> SGEKDVVFLIDGSEGVRSGFPLLKDFVQRVVESLDVGPDQVRVALVQYSDRTRPEFYLNSHMDQQGVISAIRRLTLLGGPTPNTGAALEFVLRNILTSSTGSRIAEGVPQLLIVLTAEPSGDDVRGPSVVLKQGGAVPIGIGIGNADISEMQTISFIPDFAVAIPTFRELGTIQQVISERVIQLNREELSSLKPILTPSTGAG

Collagen VI is a ubiquitously expressed extracellular matrix protein that forms a structurally unique network of beaded microfilaments. All collagen VI chains consist of a relatively short triple-helical region as well as of N- and C-terminal globular structures that are largely made up of VWA domains. Von Willebrand factor A (VWA) domains consist of about 200 amino acid residues and act as interaction modules in many intra- and extracellular proteins, e.g., in copines, integrins, von Willebrand factor, complement factors B and C2, matrilins, and collagens. The collagen VI α3N5 domain structure is the first solved structure of a collagen VWA domain and differs from other VWA domains in having an extended C-terminal region comprising residues N1206–G1224.

One of these missense mutations, R1064Q in human (R1064Qh) that is located in the N5 domain, was found in an UCMD patient (Lampe et al., 2005). To gain insight into the UCMD causing mechanism of the R1064Q mutant in human, the equivalent mutation R1061Qm in mouse was inserted into the murine collagen VI α3N5 domain by mutagenesis PCR and the crystal structure of the corresponding recombinant protein was determined at 1.2 Å resolution. The overall structure of the mutant VWA domain is very similar to the wild-type collagen VI α3N5 domain with an rmsd of 0.54 Å. The most significant structural difference is around the C terminus where the α6 helix of the mutant has a small angle with respect to the wild-type leading to a 1.5 Å displacement of the helix in the C-terminal extension. Poor electron density after residue L1213 in the mutant precluded the unambiguous assignment of the remainder of the C-terminal extension residues K2014–G2024. The residue of the R1061Qm mutation is preceding the beginning of the β2 strand and is located near the N terminus. Comparison of the wild-type and mutant structures shows that the side chains of the wild-type arginine and mutant glutamine are surface exposed and are pointing in approximately opposite directions while the remainder of the local conformation is the same. The crystal packing of the R1061Qm collagen VI α3N5 domain is different from the wild-type. While the arginine residue in the wild-type is in close proximity to the α2α3 loop of the neighboring molecule, the glutamine residue of the R1061Qm mutant interacts with the C-terminal part of the adjacent molecule (data not shown). The charge difference in the mutant and the difference in crystal packing also indicate the possibility that this mutation may alter intra- or intermolecular interactions and therefore disturb the assembly of collagen VI.> SRVLLALHDRAPQLKISDDRLTVVGEKGYSMVRASHGVRKGAWYFEITVDEMPPDTAARLGWSQPLGNLQAPLGYDKFSYSWRSKKGTKFHQSIGKHYSSGYGQGDVLGFYINLPEDTISGRGSSEIIFYKNGVNQGVAYKDIFEGVYFPAISLYKSCTVSINFGPCFKYPPKDLTYRPMSDMG;> DLPMPMRFRHLKKTSKEAVGVYRSPIHGRGLFCKRN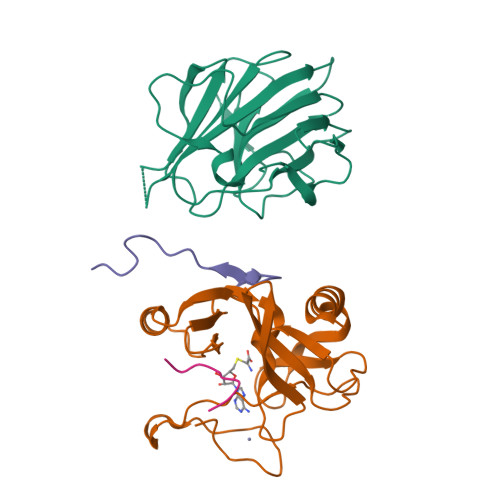IDAGEMVIEYAGIVIRSILTDKREKYYDSKGIGSSYMFRIDDSEVVDATMHGNAARFINHSCEPNCYSRVINIDGQKHIVIFAMRKIYRGEELTYDYKFPIEDASNKLPCNCGAKKCRKFLN;> SAFAPDFKELDENVEYEERESEFDIED;> ARTKQTARK> GPLGSEKPFKCSMCDYASVEVSKLKRHIRSHTGERPFQCSLCSYASRDTYKLKRHMRTHSGEKPYECYICHARFTQSGTMKMHILQKHTE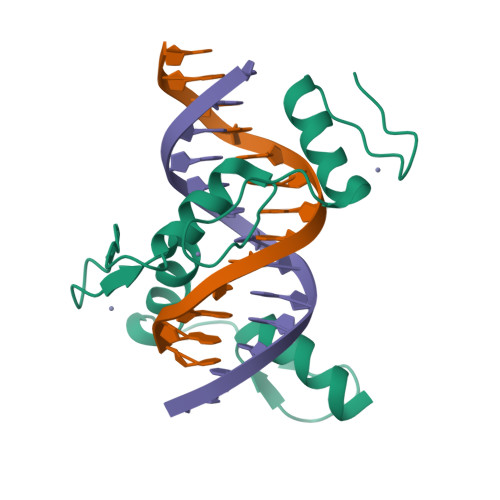NVAKFHCPHCDTVIARKSDLGVHLRKQHSYIE Latency-associated nuclear antigen (LANA) mediates γ2-herpesvirus genome persistence and regulates transcription. LANA mediates persistence of episomal DNA and thus is required for long-term maintenance of viral genomes in dividing cells, a role central to viral latency. The ORF73 from MHV-68 encodes a much smaller, 314 amino acid, 50 kDa nuclear protein (termed mLANA thereafter) which lacks the extensive internal acidic and glutamine-rich repeat region of kLANA. The C-terminal region of mLANA, comprising amino acid residues 140 to 263, has amino acid similarity to the kLANA DNA-binding domain.

The structure of the C-terminal domain of mLANA was determined at 2.2 Å resolution. The crystallized domain contained residues 140–272, designated mLANA140–272. The tertiary structure of mLANA140–272 exhibits an α+β ferredoxin-like fold which assembles to form a dimeric eight-stranded anti-parallel β-barrel that is central to its functional architecture. Each monomer contributes an anti-parallel 4-stranded β-sheet “half-barrel” from which helix α2 and α3 pack onto the plaited sheet with their axis parallel to the strands of the sheet. Size exclusion analysis confirms that mLANA140–272 is also a dimer in solution. In total, seven phosphates ions were located at the surface of mLANA. Five of these are situated on the ventral face while the remaining two cap the dorsal side of helix α1. Therefore, we consider the ventral face as the putative DNA binding site of mLANA. Electrostatic surface analysis of the mLANA protein reveals an extensive positive patch on the dorsal side which includes residues Arg-156, Lys-224, 225, 228, 229, 231, 251, 253, and Arg-232. The positive electrostatic surface also encompasses the identified 226QAKKLK231 motif that is involved in binding to BET proteins.

>[2x]GPGYQKDPPKKYQGMRRHLQVTAPRLFDPEGHPPTHFKSAVMFSSTHPYTLNKLHKCIQSKHVLSTPVSCLPLVPGTTQQCVTYYLLSFVEDKKQAKKLKRVVLAYCEKYHSSVEGTIVKAKPYFPLPEPPTEPPTDPEQP>[2x]MGSSHHHHHHPAPVEVTYKNMRFLITHNPTNATLNKFIEELKKYGVTTIVRVSEATYDTTLVEKEGIHVLDWPFDAGAPPSNQIVDDWLSLVKIKFREEPGCCIAVHCVAGLG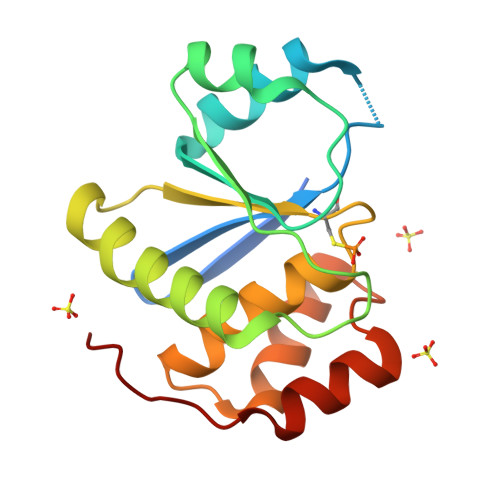RAPVLVALALIEGGMKYEDAVQFIRQKRRGAFNSKQLLYLEKYRPKMRLRF N-{(3P)-3-[(5P)-5-(2H-tetrazol-5-yl)-2,1-benzoxazol-3-yl]phenyl}cyclopentanecarboxamide | C20 H18 N6 O2 | 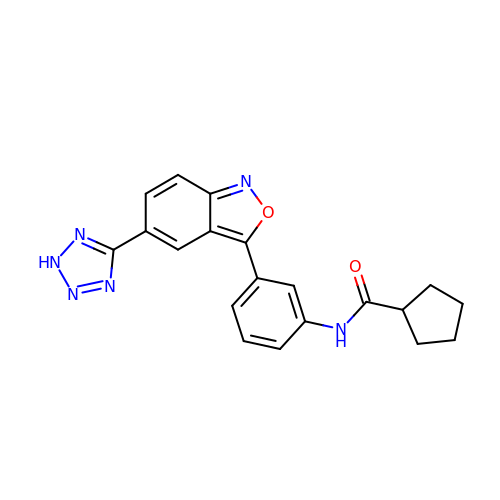OFSLXIACVHOLTC-UHFFFAOYSA-N>[3x]GSIIEMRDVVKKYDN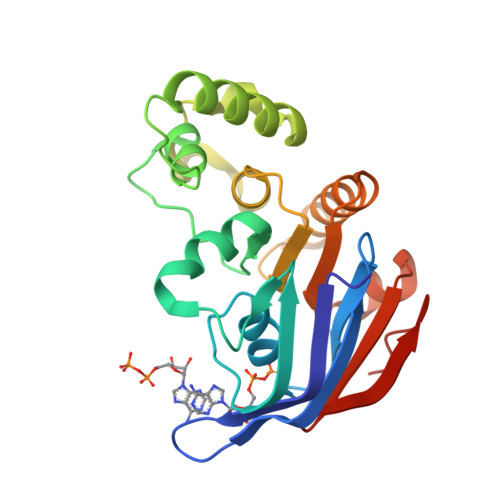GTTALRGVSVSVQPGEFAYIVGPSGAGKSTFIRSLYREVKIDKGSLSVAGFNLVKIKKKDVPLLRRSVGVVFQDYKLLPKKTVYENIAYAMEVIGENRRNIKRRVMEVLDLVGLKHKVRSFPNELSGGEQQRIAIARAIVNNPKVLIADEPTGNLDPDNSWEIMNLLERINLQGTTILMATHNSQIVNTLRHRVIAIENGRVVRDESKGEYGYDD prop-2-yn-1-yl trihydrogen diphosphate | C3 H6 O7 P2 | 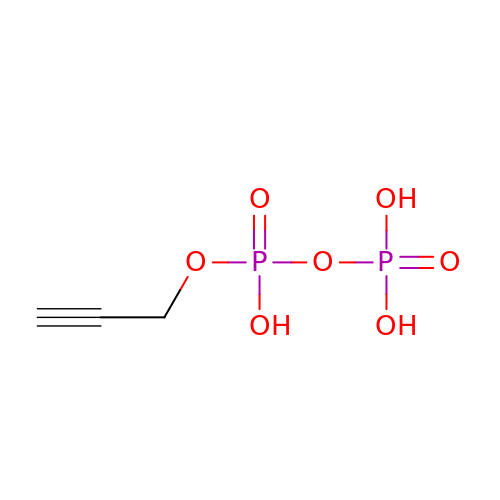CEUAGVILADDFJF-UHFFFAOYSA-N>SKAVTGMRTIDGKKYYFNTNTAEAATGWQTIDGKKYYFNTNTSIASTGYTIINDKHFYFNTDGIMQIGVFKGPDGFEYFAPANTDANNIEGQAIRYQNRFLYLHDNIYYFGNNSKAATGWVTIDGRRYYFEPNTAIGANG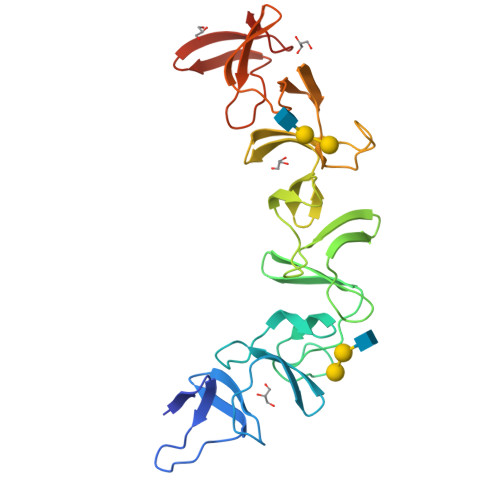YKIIDNKNFYFRNGLPQIGVFKGPNGFEYFAPANTDANNIDGQAIRYQNRFLHLLGNIYYFGNNSKAVTGWQTINGNMYYFMPDTAMAAAGGLFEIDGVIYFFGVDGVKAPGIYG[2x]> KRRWKKNFIAVSAANRFKKIS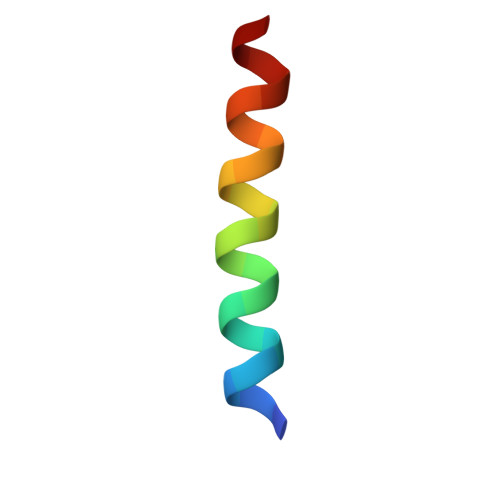S>EDENEKMFFLIDKVNAFNQDITALMQGEETVGEEDIRLFTRLRHEFHKWSTIIENNFQEGHKILSRKIQKFENQYRGRELPGFVNYRTFETIVKQQIKALEEPAVDMLHTVTDMVRLAFTDVSIKNFEEFFNLHRTAKSKIEDIRAEQEREGEKLIRLHFQMEQIVYCQDQVYRGALQKVREKELEEEKKKKSWDFGAFQSSSATDSSMEEIFQHLMAYHQEASKRISSHIPLIIQFFMLQTYGQQLQKAMLQLLQDKD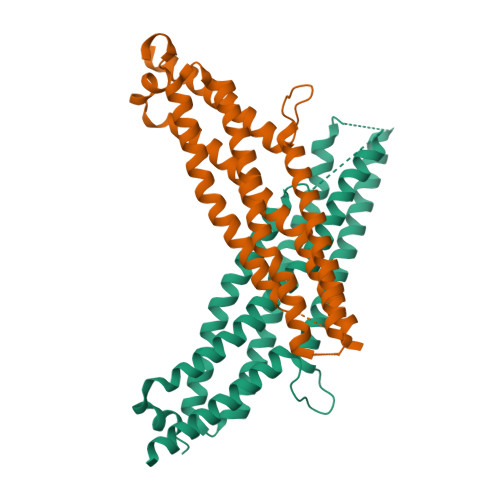TYSWLLKERSDT[2x]6-chloro-N-[(2-chlorophenyl)methyl]-1-[5-O-(phosphonomethyl)-beta-D-ribofuranosyl]-1H-pyrazolo[3,4-d]pyrimidin-4-amine 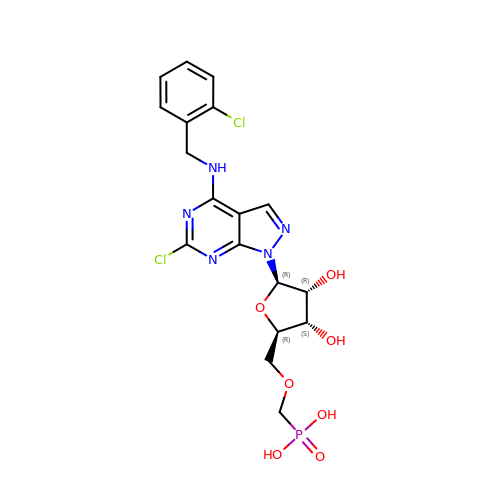| C18 H20 Cl2 N5 O7 P | VAGWGCSOWAKFTM-VMUDFCTBSA-N> MTVT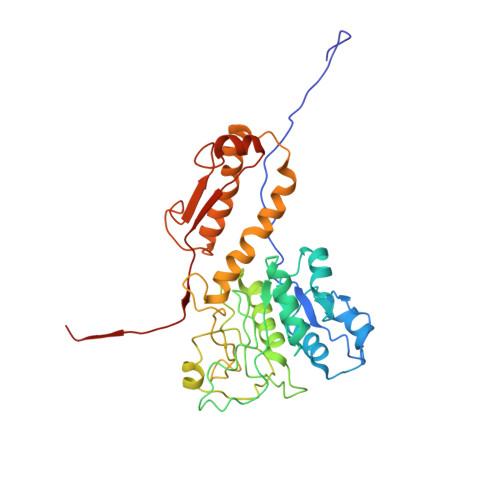TTYPGVYLSEDAVSSFSVNSAATAVPLFAYDSENTNTINKPIQVFRNWAEFTVEYPTPLEDAFYTSLSLWFMHGGGKCYLVNEANIADAVAQYDDITLIVAAGTDTTTYTAFTTVVGQGYRIFGLFDGPKEKIAGTAKPDEVMEEYPTSPFGAVFYPWGTLASGAAVPPSAIAAASITQTDRTRGVWKAPANQAVNGVTPAFAVSDDFQGKYNQGKALNMIRTFSGQGTVVWGARTLEDSDNWRYIPVRRLFNAVERDIQKSLNKLVFEPNSQPTWQRVKAAVDSYLHSLWQQGALAGNTPADAWFVQVGKDLTMTQEEINQGKMIIKIGLAAVRPAEFIILQFSQDIAQ>[8x]AEKQAKRNRREEILQSLALMLESSDGSQRITTAKLAASVGVSEAALY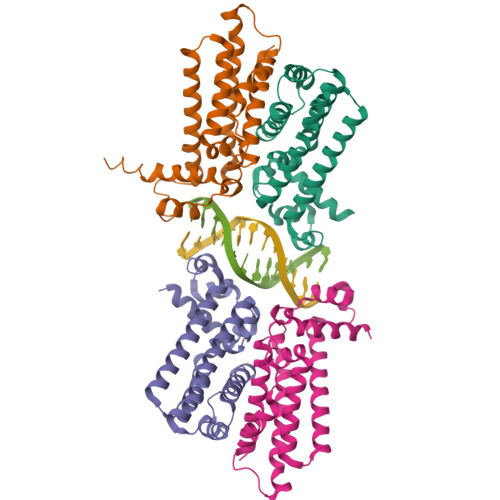RHFPSKTRMFDSLIEFIEDSLITRINLILKDEKDTTARLRLIVLLLLGFGERNPGLTRILTGHALMFEQDRLQGRINQLFERIEAQLRQVLREKRMREGEGYTTDETLLASQILAFCEGMLSRFVRSEFKYRPTDDFDARWPLIAAQLQ;> DYLDIPAFLR> GPGSCPTHADSLNNLANIKREQGNIEEAVRLYRKALEVFPEFAAAHSNLASVLQQQGKLQEALMHYKEAIRISPTFADAYSNMGNTLKEMQDVQGALQCYTRAIQINPAFADAHSNLASIHKDSGNIPEAIASYRTALKLKPDFPDAYCNLAHCLQIVCDWTDYDERMKKLVSIVADQLEKNRLPSVHPHHSMLYPLSHGFRKAIAERHGNLCLDKINVLHKPPYEHPKDLKLSDGRLRVGYVSSDFGNHPTSHLMQSIPGMHNPDKFEVFCYALSPDDGTNFRVKVMAEANHFIDLSQ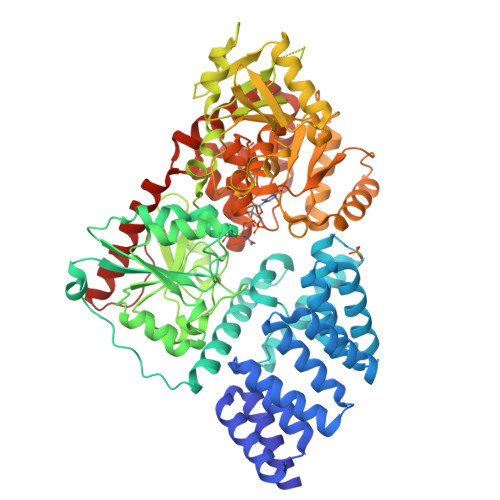IPCNGKAADRIHQDGIHILVNMNGYTKGARYELFALRPAPIQAMWLGYPGTSGALFMDYIITDQETSPAEVAEQYSEKLAYMPHTFFIGDHANMFPHLKKKAVIDFKSNGHIYDNRIVLNGIDLKAFLDSLPDVKIVKMKCPDGGDNADSSNTALNMPVIPMNTIAEAVIEMINRGQIQITINGFSISNGLATTQINNKAATGEEVPRTIIVTTRSQYGLPEDAIVYCNFNQLYKIDPSTLQMWANILKRVPNSVLWLLRFPAVGEPNIQQYAQNMGLPQNRIIFSPVAPKEEHVRRGQLADVCLDTPLCNGHTTGMDVLWAGTPMVTMPGETLASRVAASQLTCLGCLELIAKNRQEYEDIAVKLGTDLEYLKKVRGKVWKQRISSPLFNTKQYTMELERLYLQMWEHYAAGNKPDHMIKPVE> GLPVMTTPGSTQFLTSDDFQSPSAMPQFDVTPEMQIPGRVNNLMEIAEVDSVVPVNNTEDNVSSLKAYQIPVQSNSDNGKQVFGFPLQPGANNVLNRTLLGEILNYYTHWSGSIKLTFMFCGSAMATGKFLLAYSPPGAGVP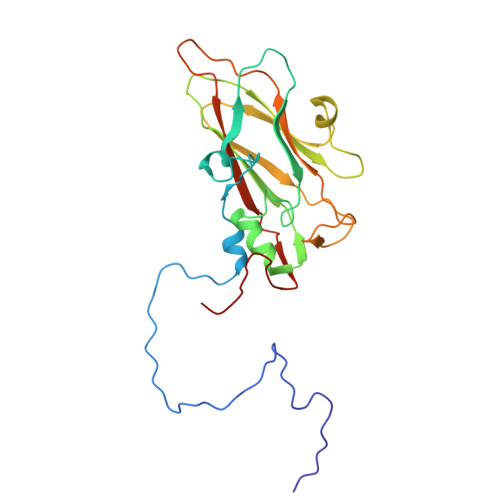KNRKDAMLGTHVIWDVGLQSSCVLCVPWISQTHYRYVVEDEYTAAGYVTCWYQTNIVVPADVQSSCDILCFVSACNDFSVRMLKDTPFIRQDTFYQ2-amino-9-(5-O-[(R)-hydroxy{[(R)-hydroxy(phosphonoamino)phosphoryl]oxy}phosphoryl]-3-O-{[2-(methylamino)phenyl]carbonyl}-beta-D-erythro-pentofuranosyl-2-ulose)-1,9-dihydro-6H-purin-6-one 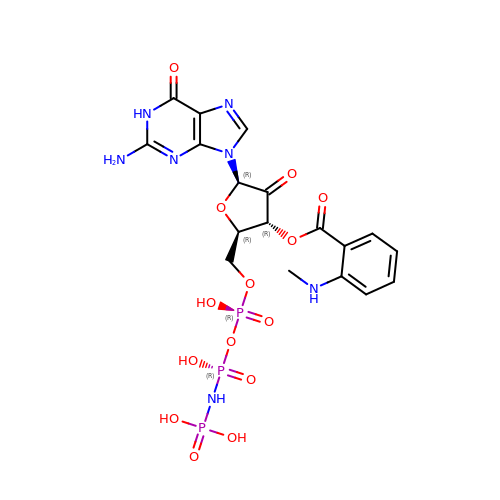| C18 H22 N7 O14 P3 | RVBPPAHXMWBKDD-CKUKBARFSA-N> MGSSHHHHHHSSGLEVLFQGPASNKVYEKTGDSVIVKVQHKETGGPRLVRLQVMGDKLIHVSATADSKFADPQSLIVVPQKKQTSFAVVQNGDTITVSTEEVKASVLASTGEVWFTDKNGELILQENKGGGKTFTPIEVEGTKGYTVCQVFESPEDEAFYGLGQHQADEFNYKGKNEELFQYNTKVSVPFVVSNKNYGILLDSYSFCRFGNPNDYSQLNRIFKLYDKTGQEGALTGTYVPKKGETLVRREDSIYFENLKTIENLPKKLPLMGAKVTYEGEIEPAQTGEFKFILYYAGYVKVYLNNEPVVPERWRTAWNPNSYKFAAHLEAGKRVPLKIEWQPDGGQSYCGLRALTPVNPEEQGKQSWWSEMTKQLDYYFMAGENMDDVISGYRSLTGKSPVMPKWAMGFWQSREKYNTQEEMLGALKGFRDRKIPLDNIVLDWNHWPENAWGSHEFDKARFPDPKAMVDSIHAMHARMMISVWPKFYVTTEHFKEFDENGWMYQQSVKDSLKDWVGPGYHYGFYDAYDPDARKLFWKQMYEHYYPLGIDAWWMDASEPNVRDCTDLEYRKALCGPTALGSSTEFFNAYALMNAEAIYDG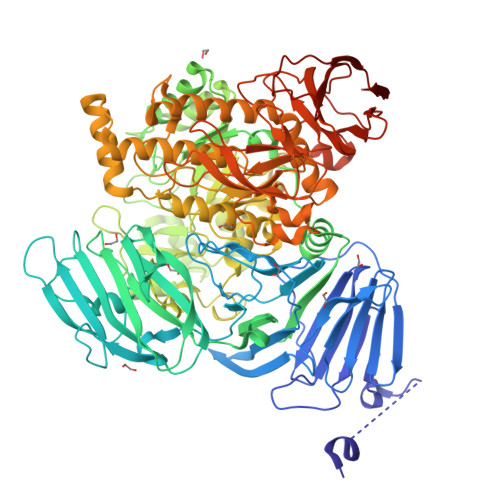QRGVDNNKRVFLLTRSGFAGLQRYSTATWSGDIGTRWEDMKAQISAGLNFAMSGIPYWTMDIGGFCVENRYVAGQKQWNATKTENADYKEWRELNTRWYQFGAFVPLYRAHGQYPFREIWEIAPEGHPAYQSVVYYTKLRYNMMPYIYSLAGMTWFDDYTIMRPLVMDFTADAEVNDIGDQFMFGPSFMVSPVYRYGDRSREIYFPQAEGWYDFYSGKFQAGGERKVIEAPYERIPLYVRAGAIIPFGDDIQYTDEKPAEHIRLYIYQGADGEFTLYEDEGVNYNYEQGMYAMIPMKYDEATKTLVIGERQGEFPGMLKERTFTVVTVNKEKAQPFDLNAKGVTVKYNGSEQTLKL> MAWPKVQPEVNIGVVGHVDHGKTTLVQAITGIWTSKHSEELKRGMTIKLGYAETNIGVCESCKKPEAYVTEPSCKSCGSDDEPKFLRRISFIDAPGHEVLMATMLSGAALMDGAILVVAANEPFPQPQTREHFVALGIIGVKNLIIVQNKVDVVSKEEALSQYRQIKQFTKGTWAENVPIIPVSALHKINIDSLIEGIEEYIKTPYRDLSQKPVMLVIRSFDVNKPGTQFNELKGGVIGGSIIQGLFKVDQEIKVLPGLRVEKQGKVSYEPIFTKISSIRFGDEEFKEAKPGGLVAIGTYLDPSLTKADNLLGSIITLADAEVPVLWNI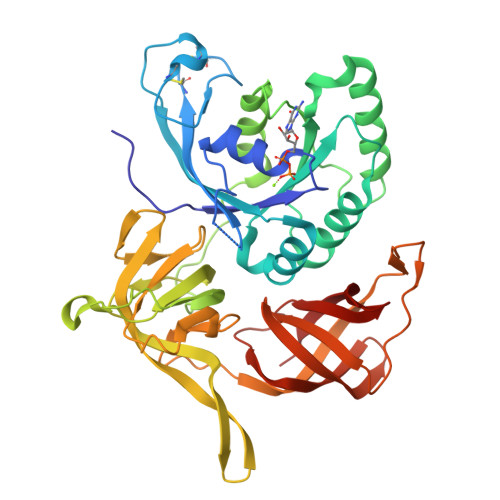RIKYNLLERVVGAKEMLKVDPIRAKETLMLSVGSSTTLGIVTSVKKDEIEVELRRPVAVWSNNIRTVISRQIAGRWRMIGWGLVEI(2E)-3-(3-chloro-4-hydroxyphenyl)prop-2-enoic acid | C9 H7 Cl O3 | 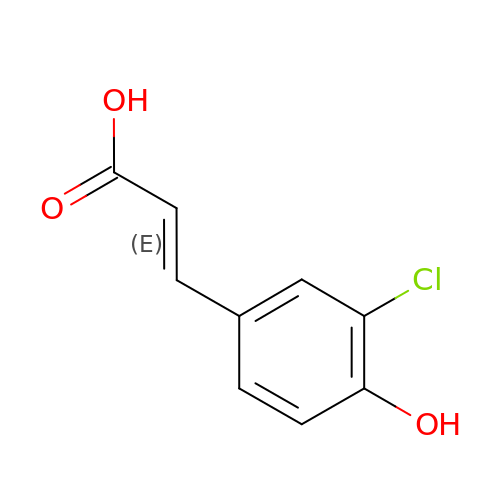VOTXWNQLOVWHNB-DUXPYHPUSA-N>[2x]MLT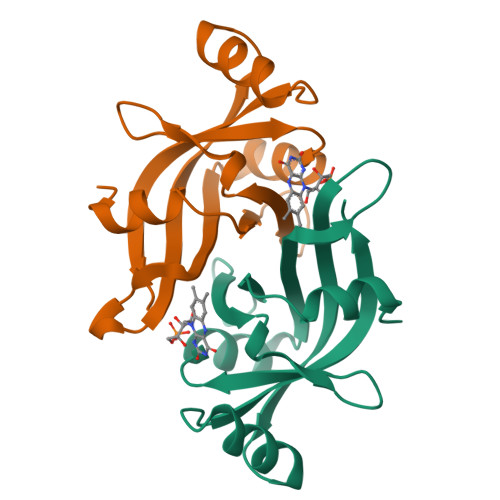KKFKETLKYEGSVSLTSWGAEKSPHVTGTWISYLQLTSDERILAPAAGMHYLEEDIKVNDTIYLMLGVREVEGKNGYQGIGFRVSAKAKLISNGPEFEMMKEKYPFLRAVLELTPVEVEQLL> SSSNYCNQMMKSRNLTKDRCKPVNTFVHESLADVQAVCSQKNVACKNG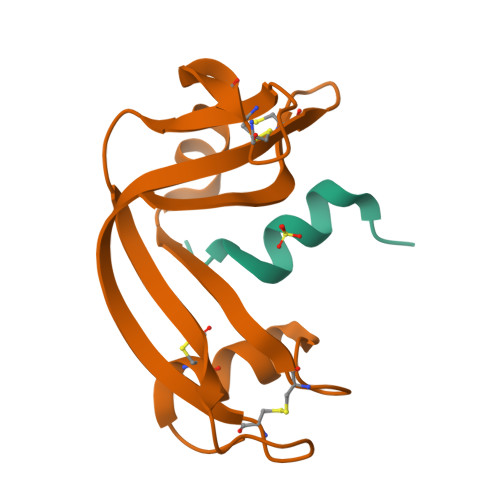QTNCYQSYSTMSITDCRETGSSKYPNCAYKTTQANKHIIVACEGNPYVPVHFDASV;> KETAAAKFERQHADSX> DCHLSDMLQQLHSVNASKPSERGLVRQEEAEDPACIPIFWVSKWVDYSDKYGLGYQLCDNSVGVLFNDSTRLILYNDGDSLQYIERDGTESYLTVSSHPNSLMKKITLLKYFRNYMSEHLLKAGANITPREGDELARLPYLRTWFRTRSAIILHLSNGSVQINFFQDHTKLILCPLMAAVTYIDEKRDFRTYRLSLLEE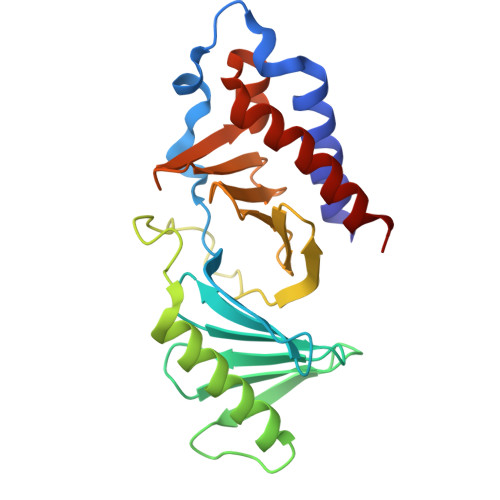YGCCKELASRLRYARTMVDKLLSS> GMHLKEKITTIIQGQRTGVLSTVRNDKPHSAFMMFFHEDFVLYVATDRQSKKITDIENNPNVHVLLGREGKKLDEDYIEVEGLASIEEDSTL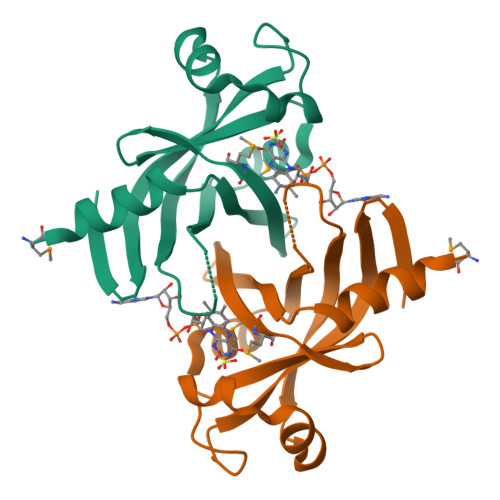KNKFWNNSLKRWLLRPEDPNYVLIKINPDTIYYIDGAGTTEPEFLRL> GAMGRILFLTTFMSKGNKVVRYLESLHHEVVISQEKVHAQSANLQEIDWIVSYAYGYILDKEIVSRFRGRIINLHPSLLPWNKGRDPVFWSVWDETPKGVTIHLIDEHVDTGDILVQEEIAFADEDTLLDCYNKANQAIEE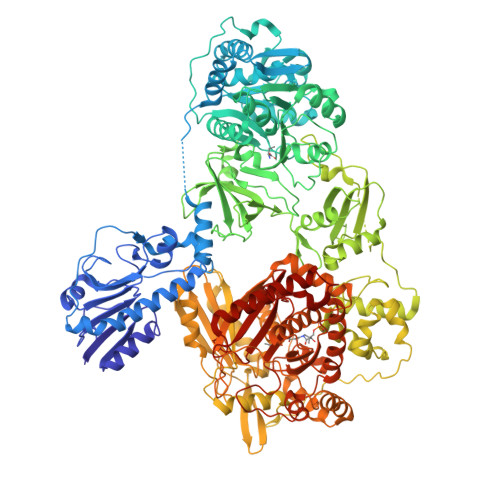LFIREWENIVHGRIAPYRQTAGGTLHFKADRDFYKNLNMTTVRELLALKRLSAEPKRGEKPIDKTFHQLFEQQVEMTPDHVAVVDRGQSLTYKQLNERANQLAHHLRGKGVKPDDQVAIMLDKSLDMIVSILAVMKAGGAYVPIDPDYPGERIAYMLADSSAAILLTNALHEEKANGASDIIDVHDPDSYSENTNNLPHVNRPDDLVYVMYTSGSTGLAKGVMIEHHNLVNFCEWYRPYFGVTPADKALVYSSFSFDGSALDIFTHLLAGAALHIVPSERKYDLDALNDYCNQEGITISYLPTGAAEQFMQMDNQSFRVVITGGDVLKKIERNGTYKLYNGYGPTECTIMVTMFEVDKPYANIPIGKPIDRTRILILDEALALQPIGVAGELFIVGEGLGRGYLNRPELTAEKFIVHPQTGERMYRTGDRARFLPDGNIEFLGRLDNLVKIRGYRIEPGEIEPFLMNHPLIELTTVLAKEQADGRKYLVGYYVAPEEIPHGELREWLGNDLPDYMIPTYFVHMKAFPLTANGKVDRRALPDVQADAELLGEDYVAPTDELEQQLAQVWSHVLGIPQMGIDDHFLERGGDSIKVMQLIHQLKNIGLSLRYDQLFTHPTIRQLKRLLTEQKQVSLEPLRELDEQAEYETSAVEKCMYIIQQQDVESIAYNVVYTINFPLTVDTEQIRVALEQLVLRHEGLRSTYHMRGDEIVKRIVPRAELSFVRQTGEEESVQSLLAEQIKPFDLAKAPLLRAGVIETADKKVLWFDSHHILLDGLSKSILARELQALLGQQVLSPVEKTYKSFARWQNEWFASDEYEQQIAYWKTLLQGELPAVQLPTKKRPPQLTFDGAIQMYRVNPEITRKLKATAAKHDLTLYMLMLTIVSIWLSKMNSDSNQVILGTVTDGRQHPDTRELLGMFVNTLPLLLSIDHEESFLHNLQQVKAKLLPALQNQYVPFDKILEAARVKREGNRHPLFDVMFMMQGAPETELESNMHHINAGISKFDLTLEVLERENGLNIVFEYNTHLFDEGMILRMVAQFEHLLLQAVHGLDQQVKRFELVAAAENLYFQ> MGSDKIHHHHHHMDAAKDDLEHAKHDLEHGFYNWACFSSQQAAEKAVKAVFQRMGAQAWGYSVPDFLGELSSRFEIPEELMDHALELDKACIPTRYPDALPSGSPRNRYSRIEA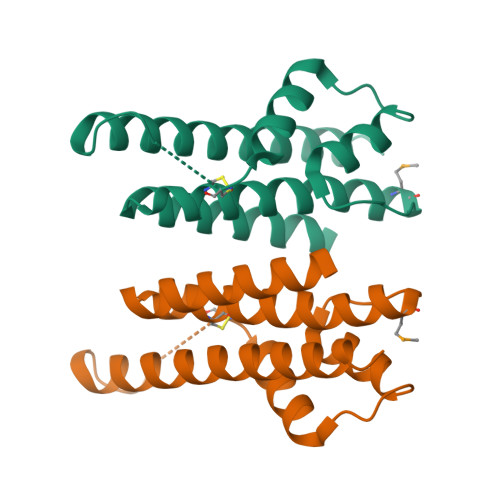ERLVNYAEKIIRFCEDLLSRI>[2x]MNPAAEAEFNILLATDSYKVTHYKQYPPNTSKVYSYFECREKKTENSKLRKVKYEETVFYGLQYILNKYLKGKVVTKEKIQEAKDVYKEHFQDDVFNEKGWNYILEKYDGHLPIEIKAVPEGFVIPRGNVLFTVENTDPECYWL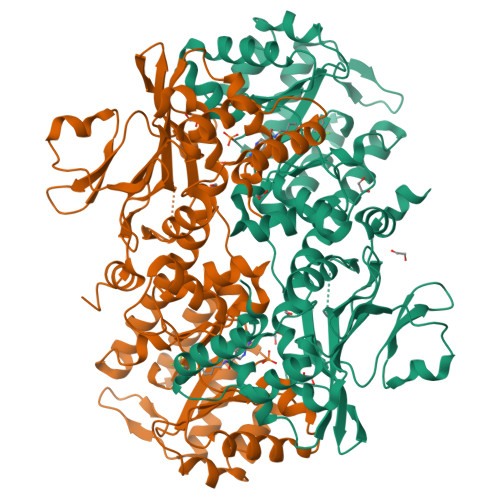TNWIETILVQSWYPITVATNSREQKKILAKYLLETSGNLDGLEYKLHDFGYRGVSSQETAGIGASAHLVNFKGTDTVAGLALIKKYYGTKDPVPGYSVPAAEHSTITAWGKDHEKDAFEHIVTQFSSVPVSVVSDSYDIYNACEKIWGEDLRHLIVSRSTQAPLIIRPDSGNPLDTVLKVLEILGKKFPVTENSKGYKLLPPYLRVIQGDGVDINTLQEIVEGMKQKMWSIENIAFGSGGGLLQKLTRDLLNCSFKCSYVVTNGLGINVFKDPVADPNKRSKKGRLSLHRTPAGNFVTLEEGKGDLEEYGQDLLHTVFKNGKVTKSYSFDEIRKNAQLNIELEAAHHLEHHHHHHHH> MDILLVCLRFPFFSVAKRSYQVRTSFLLPPPSALKGALAKGLILLKPEKYASSSLDEAALKAIKEIESKLVDIKAVSVAPLSPLIRNAFLLKRLRNLESGSNAEKSDAMRREYTFTRELLVAYIFKNLTQEEKNLYLKAAMLIDVIGDTESLATPVWASFVKPEDKKAPLAFSAPYTEIYSLLSSKIQAKGKIRMYIEKMRVSPEYSKTKGPQEEIFYLPIEERRYKRIVYYARIYPPE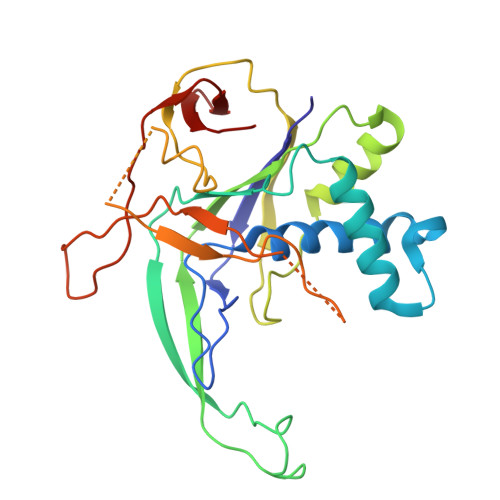VEKALTVDGEVLGIWIP> GGGRMAAATGLEEAVAPMGALCGLVQDFVMGQQEGPADQVAADVKSGGYTVLQVVEALGSSLENAEPRTRARGAQLLSQVLLQCHSLLSEKEVVHLILFYENRLKDHHLVVPSVLQGLRALSMSVALPPGLAVSVLKAIFQEVHVQSLLQVDRHTVFSIITNFMRSREEELKGLGADFTFGFIQVMDGEKDPRNLLLAFRIVHDLISKDYSLGPFVEELFEVTSCYFPIDFTPPPNDPYGIQREDLILSLRAVLASTPRFAEFLLPLLIEKVDSEILSAKLDSLQTLNACCAVYGQKELKDFLPSLWASIRREVFQTASERVEAEGLAALHSLTACLSCSVLRADAEDLLGSFLSNILQDCRHHLCEPDMKLVWPSAKLLQAAAGASARACEHLTSNVLPLLLEQFHKHSQSNQRRTILEMILGFLKLQQKWSYEDRDERPLSSFKDQLCSLVFMALTDPSTQLQLVGIRTLTVLGAQPGLLSAEDLELAVGHLYRLTFLEEDSQSCRVAALEASGTLATLYPGAFSRHLLPKLAEELHKGESDVARADGPTKCSRHFRCLQALSAVSTHPSIVKETLPLLLQHLCQANKGNMVTESSEVVAVCQSLQQVAEKCQQDPESYWYFHKTAVPCLFALAVQASMPEKESSVLRKVLLEDEVLAALASVIGTATTHLSPELAAQSVTCIVPLFLDGNTSFLPENSFPDQFQPFQDGSSGQRRLVALLTAFVCSLPRNVEIPQLNRLMRELLKQSCGHSCPFSSTAATKCFAGLLNKQPPGQQLEEFLQLAVGTVEAGLASES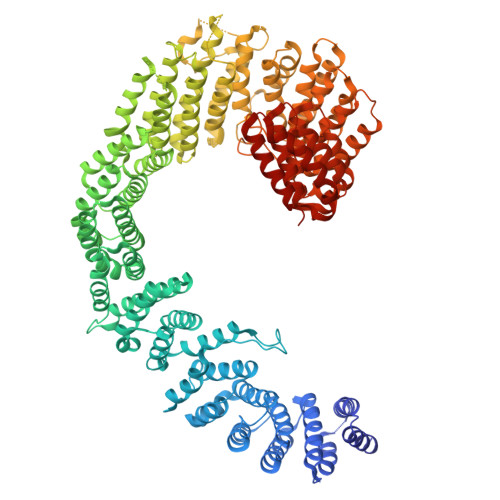SRDQAFTLLLWVTKALVLRYHPLSACLTTRLMGLLSDPELGCAAADGFSLLMSDCTDVLTRAGHADVRIMFRQRFFTDNVPALVQGFHAAPQDVKPNYLKGLSHVLNRLPKPVLLPELPTLLSLLLEALSCPDSVVQLSTLSCLQPLLLEAPQIMSLHVDTLVTKFLNLSSSYSMAVRIAALQCMHALTRLPTSVLLPYKSQVIRALAKPLDDKKRLVRKEAVSARGEWFLLGSPGS> MITTPLVHVASVEKGRSYEDFQKVYNAIALKLREDDEYDNYIGYGPVLVRLAWHISGTWDKHDNTGGSYGGTYRFKKEFNDPSNAGLQNGFKFLEPIHKEFPWISSGDLFSLGGVTAVQEMQGPKIPWRCGRVDTPEDTTPDNGRLPDADKDAGYVRTFFQRLNMNDREVVALM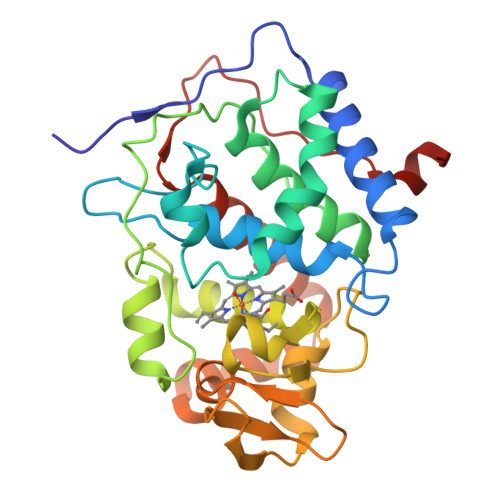GAHALGKTHLKNSGYEGPWGAANNVFTNEFYLNLLNEDWKLEKNDANNEQWDSKSGYMMLPTNYSLIQDPKYLSIVKEYANDQDKFFKDFSKAFEKLLENGITFPKDAPSPFIFKTLEEQGL>MVPISPIETVPVKLKPGMDGPKVKQWPLTEEKIKALVEICTEMEKEGKISKIGPENPYNTPVFAIKKKDSTKWRKLVDFRELNKRTQDFWEVQLGIPHPAGLKKKKSVTVLDVGDAYFSVPLDEDFRKYTAFTIPSINNETPGIRYQYNVLPQGWKGSPAIFQSSMTKILEPFKKQNPDIVIYQYMDDLYVGSDLEIGQHRTKIEELRQHLLRWGLTTPDKKHQKEPPFLWMGYELHPDKWTVQPIVLPEKDSWTVNDICKLVGKLNWASQIYPGIKVRQLSKLLRGTKALTEVIPLTEEAELELAENREILKEPVHGVYYDPSKDLIAEIQKQGQGQWTYQIYQEPFKNLKTGKYARMRGAHTNDVKQLTEAVQKITTESIVIWGKTPKFKLPIQKETWETWWTEYWQATWIPEWEFVNTPPLVKLWYQLEKEPIVGAETFYVDGAANRETKLGKAGYVTNKGRQKVVPLTNTTNQKTELQAIYLALQDSGLEVNIVTDSQYALGIIQAQPDKSESELVNQIIEQLIKKEKVYLAWVPAHKGIGGNEQVDKLVSAG[4x];>MAHHHHHHALEVLFQGPISPIETVPVKLKPGMDGPKVKQWPLTEEKIKALVEICTEMEKEGKISKIGPENPYNTPVFAIKKKDSTKWRKLVDFRELNKRTQDFWEVQLGIPHP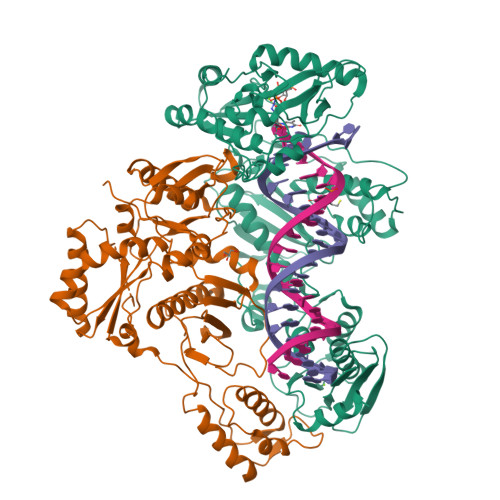AGLKKKKSVTVLDVGDAYFSVPLDEDFRKYTAFTIPSINNETPGIRYQYNVLPQGWKGSPAIFQSSMTKILEPFKKQNPDIVIYQYMDDLYVGSDLEIGQHRTKIEELRQHLLRWGLTTPDKKHQKEPPFLWMGYELHPDKWTVQPIVLPEKDSWTVNDIQKLVGKLNWASQIYPGIKVRQLSKLLRGTKALTEVIPLTEEAELELAENREILKEPVHGVYYDPSKDLIAEIQKQGQGQWTYQIYQEPFKNLKTGKYARMRGAHTNDVKQLTEAVQKITTESIVIWGKTPKFKLPIQKETWETWWTEYWQATWIPEWEFVNTPPLVKLWYQ[4x]> SMSESSARTEMKI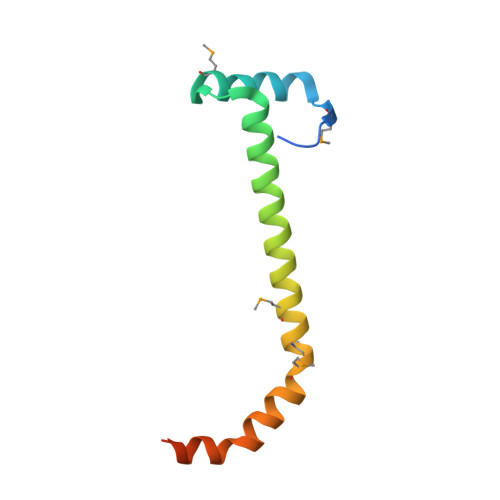SLPENLVAELDGVAMREKRSRNELISQAVRAYVSERTTRHNRDLMRRGYMEMAKINLNISSEAHFAECEAETTVERLVSGG>VNPCCYYPCQHQGICVRFGLDRYQCDCTRTGYSGPNCTIPEIWTWLRTTLRPSPSFIHFLLTHGRWLWDFVNATFIRDTLMRLVLTVRSNLIPSPPTYNIAHDYISWESFSNVSYYTRILPSVPRDCPTPMGTKGKKQLPDAEFLSRRFLLRRKFIPDPQGTNLMFAFFAQHFTHQF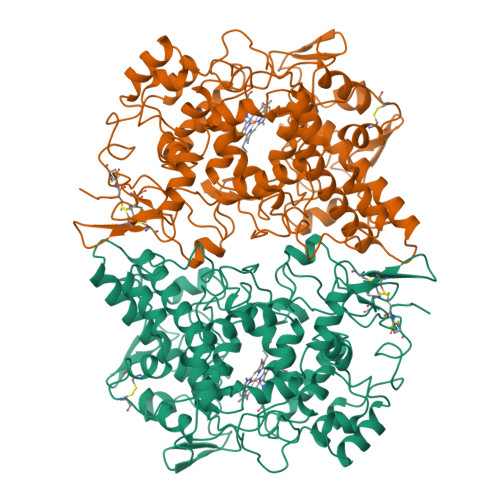FKTSGKMGPGFTKALGHGVDLGHIYGDNLERQYQLRLFKDGKLKYQMLNGEVYPPSVEEAPVLMHYPRGIPPQSQMAVGQEVFGLLPGLMLYATIWLREHQRVCDLLKAEHPTWGDEQLFQTAKLILIGETIKIVIEEYVQQLSGYFLQLKFDPELLFGAQFQYRNRIAMEFNQLYHWHPLMPDSFRVGPQDYSYEQFLFNTSMLVDYGVEALVDAFSRQPAGRIGGGRNIDHHILHVAVDVIKESRVLRLQPFNEYRKRFGMKPYTSFQELTGEKEMAAELEELYGDIDALEFYPGLLLEKCHPNSIFGESMIEMGAPFSLKGLLGNPICSPEYWKASTFGGEVGFNLVKTATLKKLVCLNTKTCPYVSFHVPDPR[2x]[(3S)-1-hydroxy-2,5-dioxopyrrolidin-3-yl]phosphonic acid 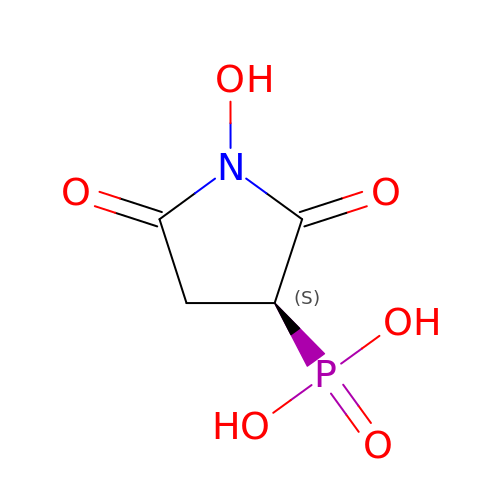| C4 H6 N O6 P | DIVWAHZZQUETIB-REOHCLBHSA-N> ISGGDAIYSSTGRCSLGFNVRSGSTYYFLTAGHCTDGATTWWANSARTTVLGTTSGSSFPNNDYGIVRYTNTTIPKDGTVGGQDITSAANATVGMAVTRRGSTTGTHSGSVTALNATVNYGGGDVVYGMIRTNVCAEPGDSGGPLYSGTRAIGLTSGGSGNCSSGGT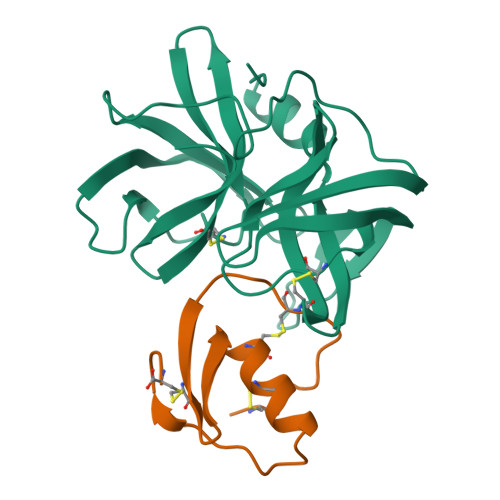TFFQPVTEALVAYGVSVY;> LAAVSVDCSEYPKPACTLEYRPLCGSDNKTYGNKCNFCNAVVESNGTLTLSHFGKC>MKLTASLTLLTQALAVLGADTNSWKSRTIYFALTDRVARSASDNGGDGCGQLQDYCGGTFKGLEGKLDYIKGMGFDAIWITPVVQNSARGYHGYWASNLYATNSHYGTSDELKGLVNAAHGKGIYIMVDVVANHVGNGPLNEMQPAPLNQGSSYHPACGINYNDQHSIETCRVASDLPDLDTTDPKIRTLYKDWIKWLMSTYKFDGVRIDTVKHVEKDFWPDFAWASGSYTIGEVFSGDPNYVAGYSKLMGGLLNYPVYFPLNRFYQQQNSSQALVDMHNQIGSLVPDPTTLGTFLDNHDNPRFLSQKNDVSLFKNALTYVLLARGIPIVYYGSEQAYAGGGDPQNREDLWRSRFNT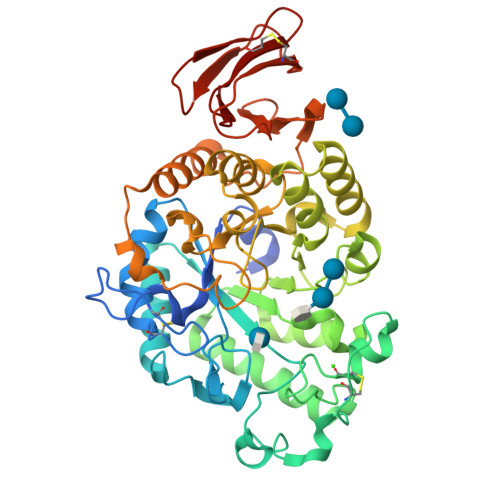NSDMYKFFQALGGVRKSHGGLPGNDHVHLFVESDAYAWSRQDGAVMALTSNIGKGQQRQFCFFTQKNNKTWRGIFDGKTYTSGGDGKLCATVNNGEPIVFVAQ[2x]(2~{R})-2-(2-chlorophenyl)-2-oxidanyl-ethanenitrile | C8 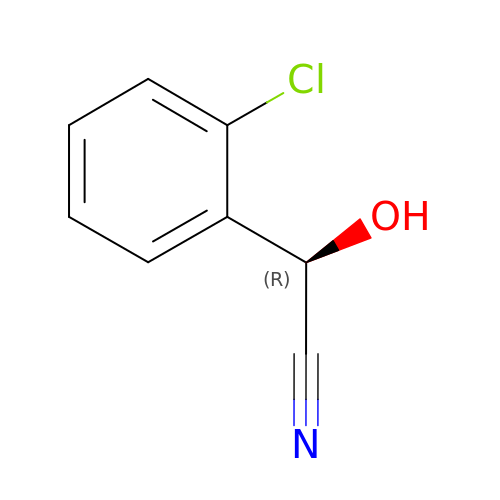H6 Cl N O | ZECLJEYAWRQVIB-QMMMGPOBSA-N>[2x]MSEAGNVASGLGLPGEVSQWSLKRYGRFMLLDNVGSPGPSSEAAAAGSSTWKVFESSEE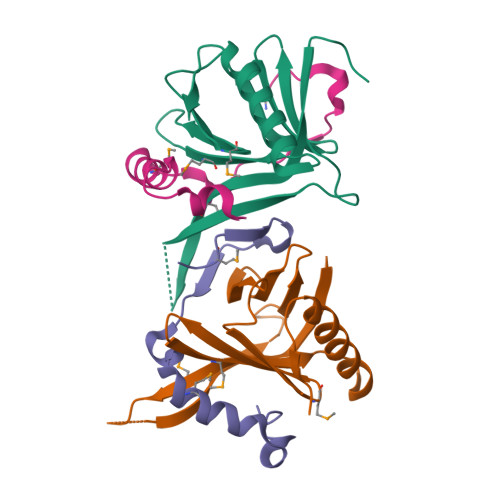SGSLVLTIVVSGHFFISQGQTLLEGFSLIGSKNWLKIVRRMDCLLFGTTIKNKSRMFRVQFSGESKEEALERCCGCVQTLAQYVTVQEPDSTTQELQQS;>[2x]SSRESMQTIPHYLQIKEILQISKQELLPCHVMEQHWKFYVGRSHSEALLSW>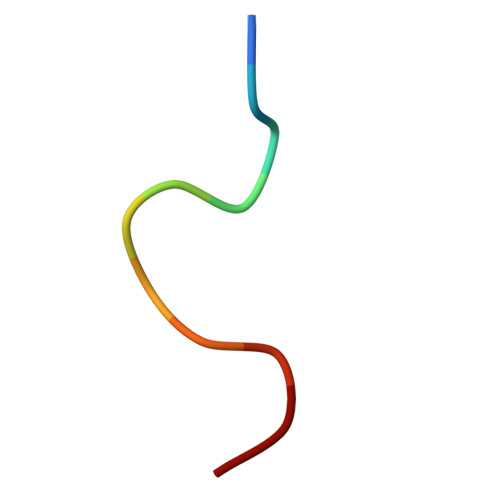 YDPFKGSDPFA>GMEVNRLSALTPPMGWNSWDCYGASVTEEEVLGNAEYMANHLKKYGWEYIVVDIQWYEPTANSSAYNPFAPLCMDEYGRLLPATNRFPSAKNGAGFKPLSDAIHDLGLKFGIHIMRGIPRQAVYENSPVLGSTKTAREIAHTNSICPWNTDMYGVDPTKEGAQSYYNSLFELYAQWGVDFVKVDDIAASRLYDTHLEEIKMIQRAIQACGRPMVLSLSPGPAPIKYAHHFKTNANMWRITDDFWDDWSLLYQMFERCEVWEKHIGTGHWPDCGMLPLGHIGIRSVDGPGGDRWTRFTKDEQLTMMNLWAICHSPLMFGGELRDNDEWTLSLLTNEGILS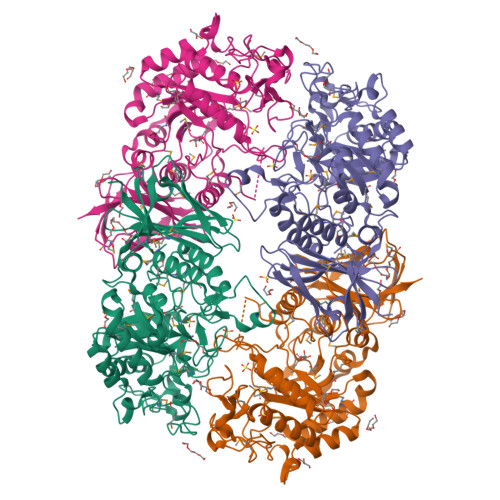INQKSVLNRFVYREEDKVAWAANGRNGEAYVALFNLHDQQKTLQFRLDMVGIMETVQLFNVWDRSFLQSLAPSESFQIELKPHQSMMLKLSPDR[2x]>[2x]GPQDNPYERGPDPTEDSIEAIRGPFSVATERVSSFAS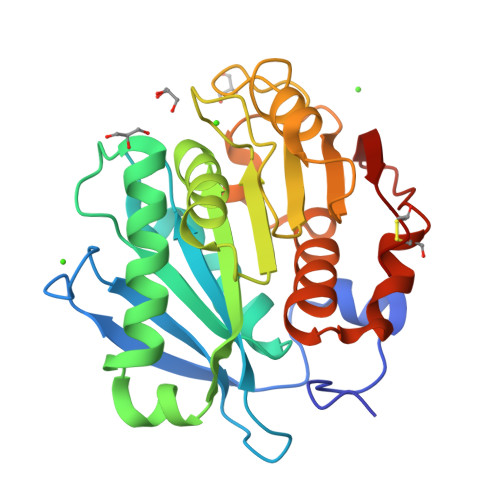GFGGGTIYYPRETDEGTFGAVAVAPGFTASQGSMSWYGERVASQGFIVFTIDTNTRLDQPGQRGRQLLAALDYLVERSDRKVRERLDPNRLAVMGHAMGGGGSLEATVMRPSLKASIPLTPWNLDKTWGQVQVPTFIIGAELDTIAPVSTHAKPFYESLPSSLPKAYMELDGATHFAPNIPNTTIAKYVISWLKRFVDEDTRYSQFLCPNPTDRAIEEYRSTCPYKLN>[2x]RSYEQMETDGERQNA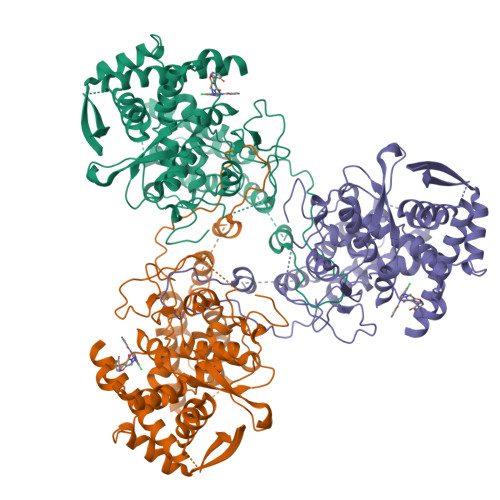TEIRASVGKMIDGIGRFYIQMCTELKLSDYEGRLIQNSLTIERMVLSAFDERRNKYLEEHPSAGKDPKKTGGPIYRRVDGKWRRELILYDKEEIRRIWRQANNGDDATAGLTHMMIWHSNLNDATYQRTRALVRTGMDPRMCSLMQGSTLPRRSGAAGAAVKGVGTMVMELIRMIKRGINDRNFWRGENGRRTRIAYERMCNILKGKFQTAAQRTMVDQVRESRNPGNAEFEDLIFLARSALILRGSVAHKSCLPACVYGSAVASGYDFEREGYSLVGIDPFRLLQNSQVYSLIRPNENPAHKSQLVWMACHSAAFEDLRVSSFIRGTKVVPRGKLSTRGVQIASNENMETMESSTLELRSRYWAIRTRSGGNTNQQRASSGQISIQPTFSVQRNLPFDRPTIMAAFTGNTEGRTSDMRTEIIRLMESARPEDVSFQGRGVFELSDEKATSPIVPSFDMSNEGSYFFGDNAEEYDNLEHHHHHH> GSKSTFLTTGQITPEEFVQAGDYLAHMFPTWKWNEESSDISYRDFLPKNKQFLIIRKVPADKRAEQAVEAKDMAQERYYDLYIAYSTSYRVPKMYIVGFNSNGSPLSPEQMFEDIS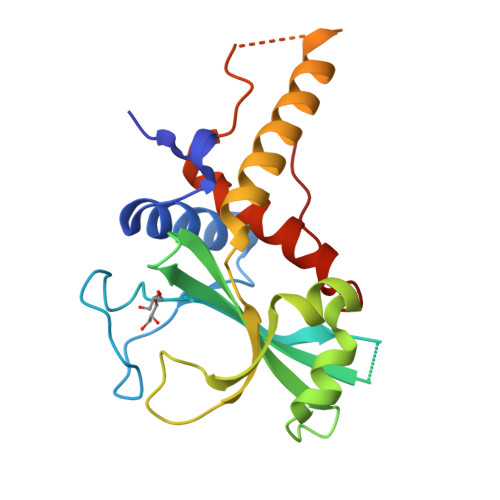ADYRTKTATIEKLPFYKNSVLSVSIHPCKHANVMKILLDKVRVVRQRRRKELQEEQELDGVGDWEDLQDDIDDSLRVDQYLIVFLKFITSVTPSIQHDYTMEGW>GMQKTAFIWDLDGTLLDSYEAILSGIEETFAQFSIPYDKEKVREFIFKYSVQDLLVRVAEDRNLDVEVLNQVRAQSLAEKNAQVVLMPGAREVLAWADESGIQQFIYTHKGNNAFTILKDLGVESYFTEILTSQSGFVRKPSPEAATYLLDKYQLNSDNTYYIGDRTLDVEFAQNS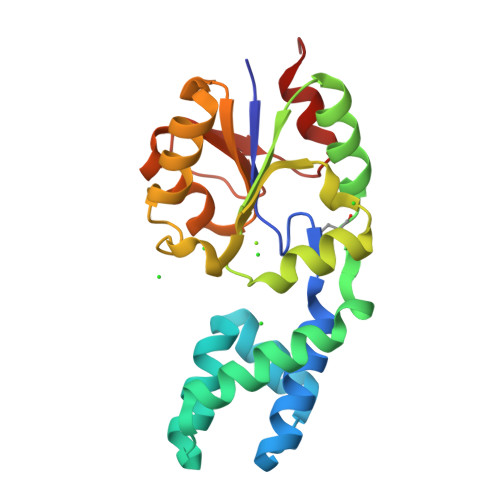GIQSINFLESTYEGNHRIQALADISRIFETK[4x]> IIGGQKAKMGNFPWQVFTNIHGRGG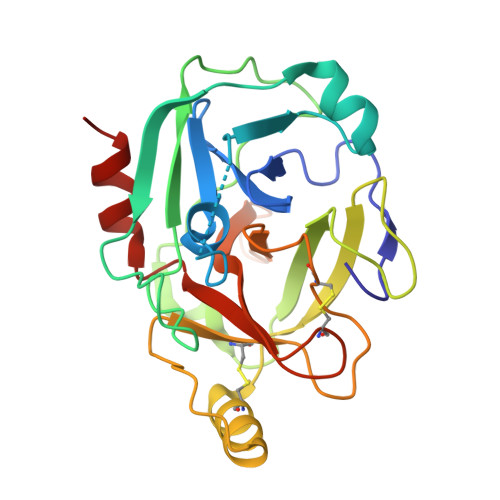GALLGDRWILTAAHTLYPKEHEAQSNASLDVFLGHTNVEELMKLGNHPIRRVSVHPDYRQDESYNFEGDIALLELENSVTLGPNLLPICLPDNDTFYDLGLMGYVSGFGVMEEKIAHDLRFVRLPVANPQACENWLRGKNRMDVFSQNMFCAGHPSLKQDACQGDSGGVFAVRDPNTDRWVATGIVSWGIGCSRGYGFYTKVLNYVDWIKKEMEEED>MADSDPGERSYDNMLKMLSDLNKDLEKLLEEMEKISVQATWMAYDMVVMRTNPTLAESMRRLEDAFLNCKEEMEKNWQELLTETKRKQ[2x]

The synaptonemal complex (SC)2 is a unique biological structure, formed through the supramolecular assembly of largely α-helical coiled-coil protein components, that binds together homologous chromosome pairs during the first meiotic division (1–3). In mammals, the SC is formed of at least eight protein components: SYCP1–3, SYCE1–3, TEX12, and SIX6OS1. SYCE3 is a small protein of 88 amino acids that is essential for SC assembly, meiotic division, and fertility. Thus, the role of SYCE3 as a synapsis initiation factor may be achieved by mediating SC central element interactions.

The crystal structure of mouse SYCE3 has been reported, revealing a compact four-helical bundle formed of two helix-loop-helix chains interacting in an anti-parallel configuration. The resultant structure is more complete and covers amino acids 10–85, which includes the additional loops and short N-terminal extensions. The SAXS scattering curve was poorly fitted by the crystal structure, with a χ2 value of 22.2. We reasoned that this may be due to the 9-amino acid N termini that are present at either end of the molecule but are absent from the crystal structure owing to lack of electron density. We modeled N termini onto the structure using MODELLER, with them adopting largely flexible conformations. This full-length model fitted closely to experimental SAXS data with a χ2 value of 1.46, indicating that scattering data are well-explained by the crystal structure with additional unstructured N termini. Thus, we conclude that solution-state SYCE3 adopts the compact dimeric fold observed in its crystal structure. We identified Tyr-11, Trp-41, and Trp-44 as surface aromatic residues that exhibit high crystallographic B-factors, indicating that their side chains are flexible and do not contribute to the dimer fold. The Tyr-11/Leu-15 and Trp-41/Tyr-44 interfaces from both chains are located on the same side of the SYCE3 dimer, indicating the presence of a single self-assembly surface.> 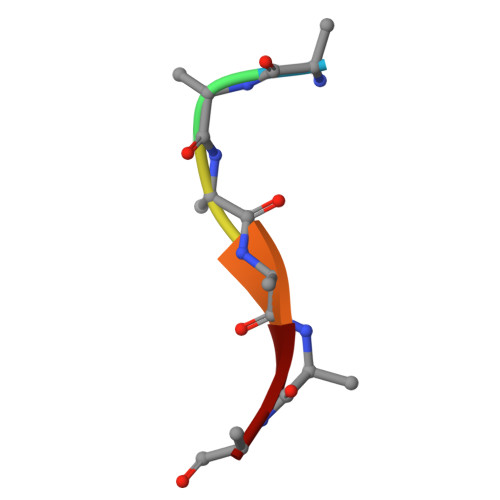AAAAAA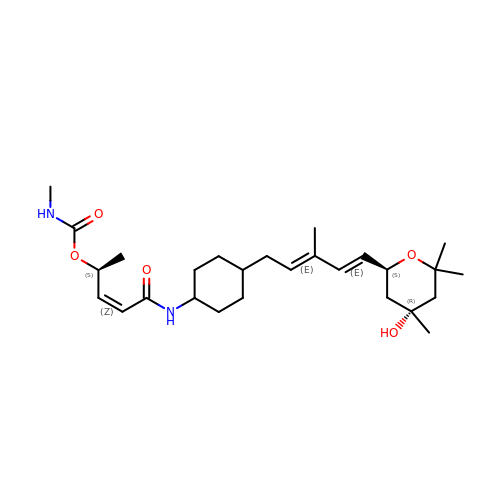[(~{Z},2~{S})-5-[[4-[(2~{E},4~{E})-3-methyl-5-[(2~{S},4~{R})-4,6,6-trimethyl-4-oxidanyl-oxan-2-yl]penta-2,4-dienyl]cyclohexyl]amino]-5-oxidanylidene-pent-3-en-2-yl] ~{N}-methylcarbamate | C27 H44 N2 O5 | WXUPGKFMAYJXHQ-PSSYVFDHSA-N> 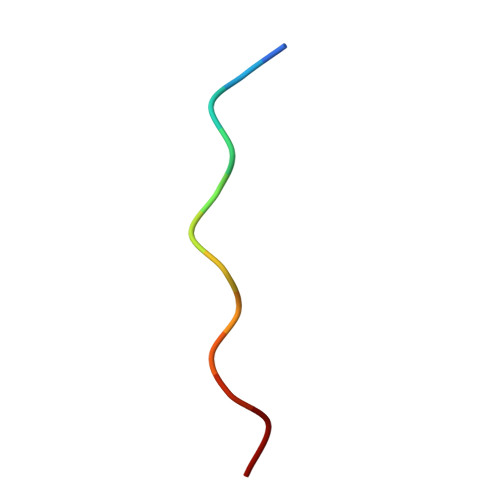AWPAWPAWPAWP>GSTYPPTPPNVTRLSDESVMLRWMVPRNDGLPIVIFKVQYRMVGKRKNWQTTNDNIPYGKPKWNSELGKSFTASVTDLK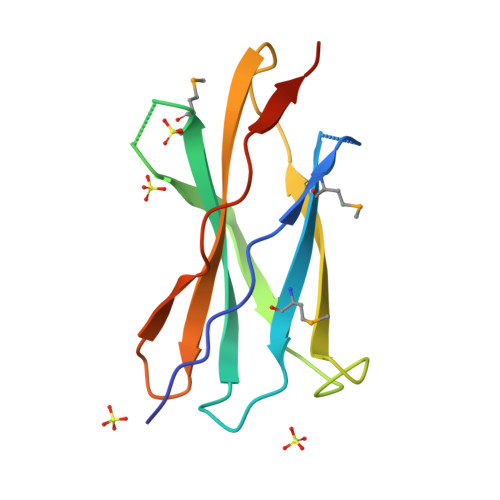PQHTYRFRILAVYSNNDNKESNTSAKFYLQPGAALD[2x]>[2x]MATAQVTCVWDLKATLGEGPIWHGDTLWFVDIKQRKIHNYHPATGERFSFDAPDQVTFLAPIVGATGFVVGLKTGIHRFHPATGFSLLLEVEDAALNNRPNDATVDAQGRLWFGTMHDGEENNSGSLYRMDLTGVARMDRDICITNGPCVSPDGKTFYHTDTLEKTIYAFDLAEDGLLSNKRVFVQFALGDDVYPDGS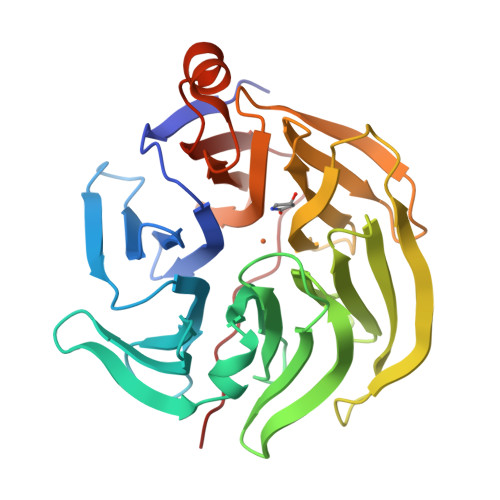VVDSEGYLWTALWGGFGAVRFSPQGDAVTRIELPAPNVTKPCFGGPDLKTLYFTTARKGLSDETLAQYPLAGGVFAVPVDVAGQPQHEVRLV> KSLLQQL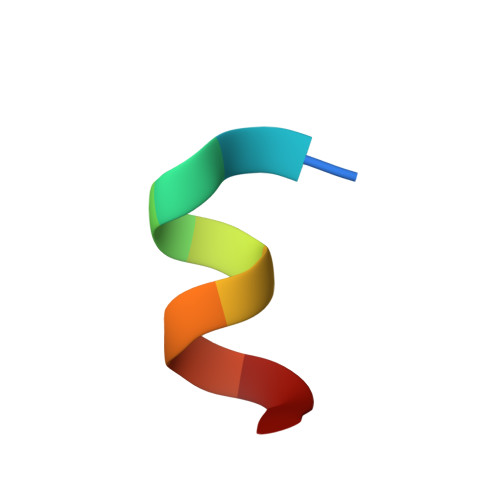LTE>[2x]EFSEDCENIFHDNAYLLKLDCEAGRVDPVEYDDISDEEIYEITVDVGVSSEDQEKVAKIIRECIAQVSTQDCTKFSEIYDCYMKKKICNYYPENMHHHHHH

Immunization with DNA plasmid coding for the salivary protein SALO (formerly known as LJM19) was shown to protect hamsters against the fatal outcome of visceral leishmaniasis and this protection was correlated with the induction of a Th1 cellular immune response. Recently, a combination vaccine comprised of recombinant salivary protein SALO and a genetically modified Leishmania donovani resulted in a strong protection against visceral leishmaniasis, further suggesting SALO as an important component for a visceral leishmaniasis vaccine. In this study we present the production and crystal structure of SALO genetically engineered in yeast as part of efforts to develop it as a recombinant vaccine for leishmaniasis. SALO is ~80% helical, has no appreciable structural similarities to any human protein, and has limited structural similarity in the C-terminus to members of insect odorant binding proteins.

Recombinant SALO was expressed as a soluble secreted protein using Pichia pastoris, rSALO(P), with yields of 1g/L and >99% purity as assessed by SEC-MALS and SDS-PAGE. The structure of rSALO(P) was solved by S-SAD at Cu-Kalpha to 1.94 Å and refined to Rfactor 17%. SALO has three predicted human CD4+ T cell epitopes on surface exposed helices. Unlike its native counterpart, rSALO(P) does not inhibit the classical pathway of complement; however, antibodies to rSALO(P) inhibit the anti-complement activity of sand fly salivary gland homogenate. Immunization with rSALO(P) produces a delayed type hypersensitivity response in C57BL/6 mice, suggesting rSALO(P) lacked anti-complement activity but retained its immunogenicity.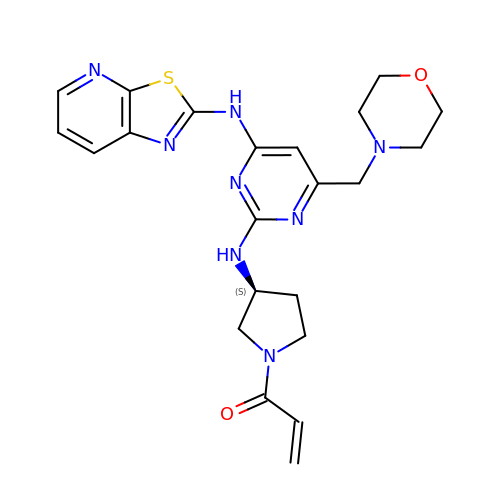1-[(3S)-3-{[4-(morpholin-4-ylmethyl)-6-([1,3]thiazolo[5,4-b]pyridin-2-ylamino)pyrimidin-2-yl]amino}pyrrolidin-1-yl]prop-2-en-1-one | C22 H26 N8 O2 S | LZANMDGKZJPQIB-HNNXBMFYSA-N>[3x]MSNSNVETFFKSSSEKNKNNFKEISCCFKISNEERSLPFQLIWSGIIIISCIGMFW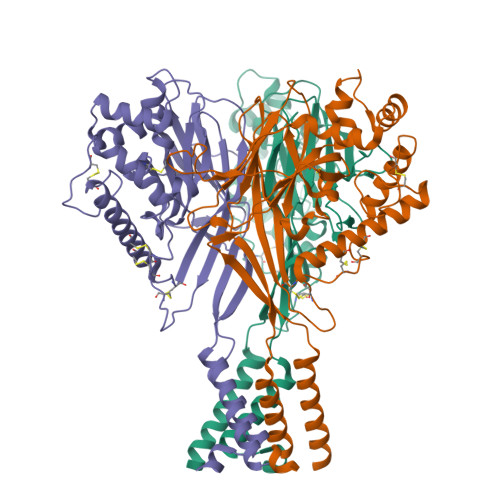NVVENIKLYFYSSPSVKFEYIKNDSLYFPAITICPFLLNWNPFFTESISFFPEMNDIFEIIETNEYDMLYLWNKTDEYFQYDDSYVYQDALIEEDEFDRSSIIPNTEIMSVSGKCHMYSLEEPVYIGNAIPNILIVYNHSKIYKDKWIKVLIHSIEDKLTSHFFAINVGVDSLLQQMTEVNFQVIQKINLNLSNNPCLFPEEVDKCFKKCLDNFMFKDLSRIHKCRLPFMDYPPDIPYCNYTNFPQMYTRFNKILKGFNKTNCLCPRKCRETRYEIQYQFNIGGFNNQTFIKITSRNSITLETEYWSYNFYSLLSDIGGSLGLFLGASILSMCEIMQKILRNFCMYSLSLKNRVLSRNSVHKINY>[2x]GSHMMAEQVALSRTQVCGILREELFQGDAFHQSDTHIFIIMGASGDLAKKKIYPTIWWLFRDGLLPENTFIVGYARSRLTVA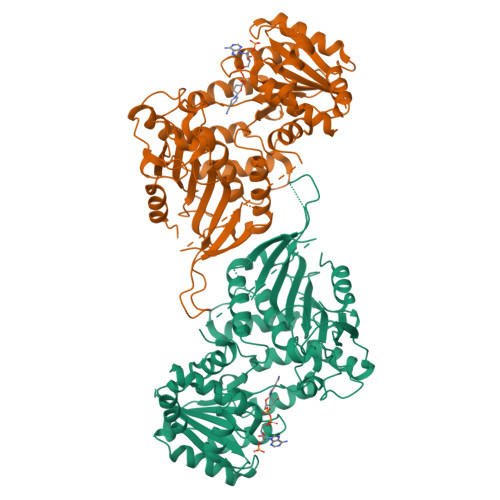DIRKQSEPFFKATPEEKLKLEDFFARNSYVAGQYDDAASYQRLNSHMNALHLGSQANRLFYLALPPTVYEAVTKNIHESCMSQIGWNRIIVEKPFGRDLQSSDRLSNHISSLFREDQIYRIDHYLGKEMVQNLMVLRFANRIFGPIWNRDNIACVILTFKEPFGTEGRGGYFDEFGIIRDVMQNHLLQMLCLVAMEKPCSTNSDDVRDEKVKVLKCISEVQANNVVLGQYVGNPDGEGEATKGYLDDPTVPRGSTTATFAAVVLYVENERWDGVPFILRCGKALNERKAEVRLQFHDVAGDIFHQQCKRNELVIRVQPNEAVYTQMMTKKPGMFFNPEESELDLTYGNRYKNVKLPDAYERLILDVFCGSQMHFVRSDELREAWRIFTPLLHQIELEKPKPIPYIYGSRGPTEADELMKRVGFQYEGTYKWVNPHKLC> LVEQEQTLE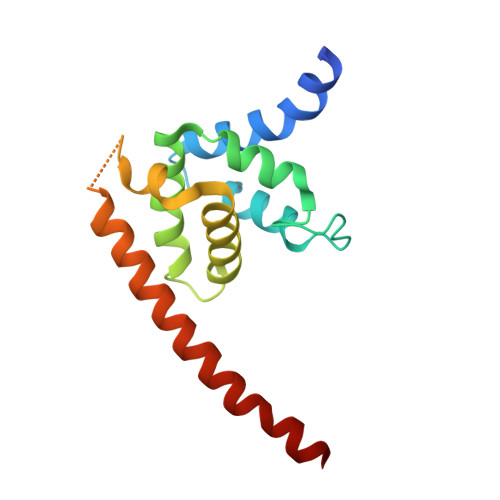NYIHAGAYRDAIVLALQLNHPGRLLNLFTNVVTTRNPDPDSLTGLKAVDDVLAKLSDEQIFQLLLRLRDWNTNARTAPVAQRVLWALFKSHPANKLSSLSVKGARGHKSLNEVLDAIKVYTERHYKRIEELVDESYLVEYTLR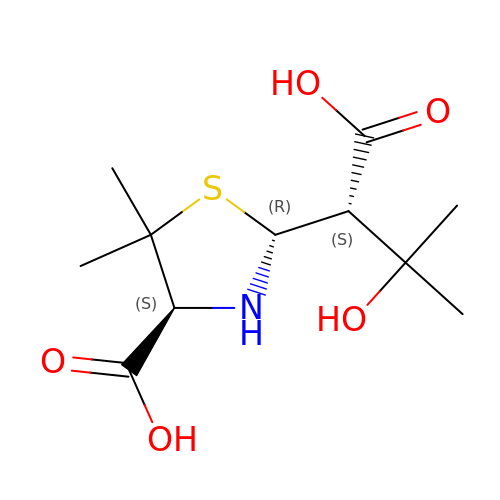2-(1-CARBOXY-2-HYDROXY-2-METHYL-PROPYL)-5,5-DIMETHYL-THIAZOLIDINE-4-CARBOXYLIC ACID | C11 H19 N O5 S | MAATUKZAHQWKEG-DSYKOEDSSA-N>[4x]DLADRFAELERRYDARLGVYVPATGTTAAIEYRADERFAFCSTFKAPLVAAVLHQNPLTHLDKLITYTSD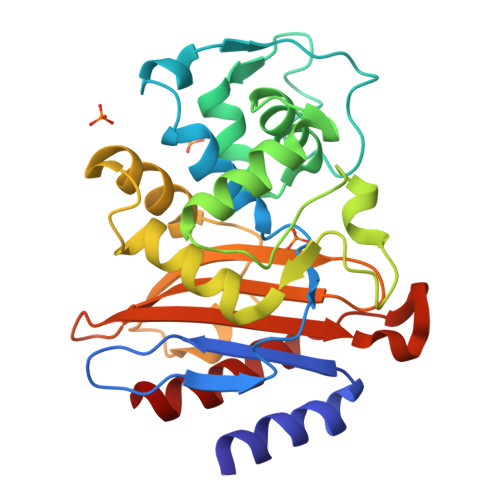DIRSISPVAQQHVQTGMTIGQLCDAAIRYSDGTAANLLLADLGGPGGGTAAFTGYLRSLGDTVSRLDAEAPELNRDPPGDERDTTTPHAIALVLQQLVLGNALPPDKRALLTDWMARNTTGAKRIRAGFPADWKVIDKTGTGDYGRANDIAVVWSPTGVPYVVAVMSDRAGGGYDAEPREALLAEAATCVAGVLA>MIVKKLTLPKDFLWGGAVAAHQVEGGWNKGGKGPSICDVLTGGAHGVPREITKEVLPGKYYPNHEAVDFYGHYKEDIKLFAEMGFKCFRTSIAWTRIFPKGDEAQPNEEGLKFYDDMFDELLKYNIEPVITLSHFEMPLHLVQQYGSWTNRKVVDFFVRFAEVVFERYKHKVKYWMTFNEINNQRNWRAPLFGYCCSGVVYTEHENPEETMYQVLHHQFVASALAVKAARRINPEMKVGCMLAMVPLYPYSCNPDDVMFAQESMRERYVFTDVQLRGYYPSYVLNEWERRGFNIKMEDGDLDVLREGTCDYLGFSYYMTNAVKAEGGTGDAISGFEGSVPNPYVKASDWGWQIDPVGLRYALCELYERYQRPLFIVENGFGAYDKVEEDGSINDDYRIDYLRAHIEEMKKAVTYDGVDLMGYTPWGCIDCVSFTTGQYSKRYGFIYVNKHDDGTGDMSRSRKKSFNWYKEVIASNGEKL[4x]

In all, we determined 23 structures, four of them not deposited in the protein data bank. These novel structures represent enzymes involved in stress response, specifically methylglyoxal reductase (YghZ), as well as three enzymes important in core metabolic functions, phosphoglucose isomerase (pGI), 6-phospho-beta-glucosidase (BglA), and glutamate dehydrogenase (GDH). All the proteins are oligomeric (YghZ, pGI, BglA, GDH) and belong to three different fold families. YghZ and BglA have a classic TIM barrel structure, pGI adopts an alpha/beta fold, and GDH possesses a core Rossmann fold found in many nucleotide binding proteins. Based on these experiments, we demonstrate successful structural characterization of multiple proteins using only microgram quantities of purified material.

6-phospho-beta-glucosidase (BglA), is a cytoplasmic enzyme and part of the glycosal hydrolase family that is able to hydrolyse aromatic β-glucoside phosphates into glucose-6-phosphate and a hydroxyl aromatic in vitro. E. coli has several predicted enzymes in this family, whose physiological role has not been fully described. BglA forms an 8-strand alpha/beta TIM barrel with the putative catalytic residues Glu180 and Glu377 located in beta strands 4 and 7. Additional density was noted in the active site and a sulfate molecule from the crystallization conditions was well ordered adjacent to the putative catalytic residues Glu180 and Glu377 and formed hydrogen bonding interactions with Thr434 and Trp425. Modeling glucose-6-phosphate into the active site based on the position of the sulfate molecule revealed residues likely involved in substrate positioning.>[2x]CT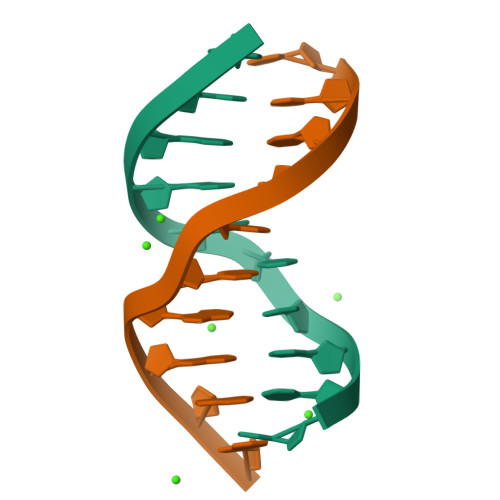CTCGAGAG>[2x]MPEDLDALLDLAARHGLDLDGGTLRTEEIGLDFRVAFARAHDGGDWVLRLPRRPDVLERAAVEGRLLAMLAPHLDVAVPDWRISTSELIAYPLLPGSPGLTVAADGEVSWHVDMASTVYARSLGSVVAQLHAVDAEAAAATGIEVRSPAQVRGAWRQDLARVGAEFEIAPALRERWEAWLADDGCWPGHSVLTHGELYPAHTLVEDERITAVLDWTTAAVGDPAKDLMFHQVSAPSAIFE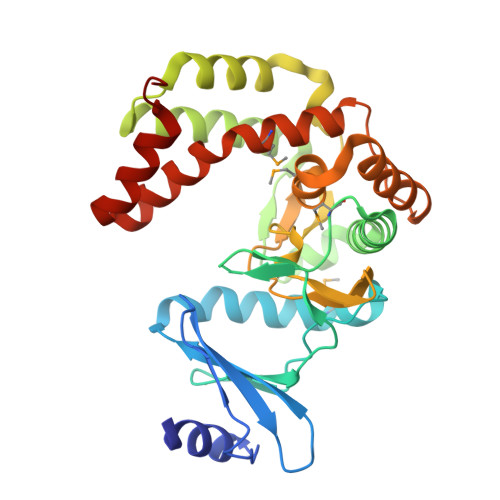VALQAYAEGGGRPWPGLARHCTEMFSAAPLGYGLYALATGEAAHREAAAAALNPPEER> FEGEKVFRVNVEDENDISELHELASTRQIDFWKPDSVTQIKPHSTVDFRVKAEDILAVEDFLEQNELQYEVLINNLRSVLE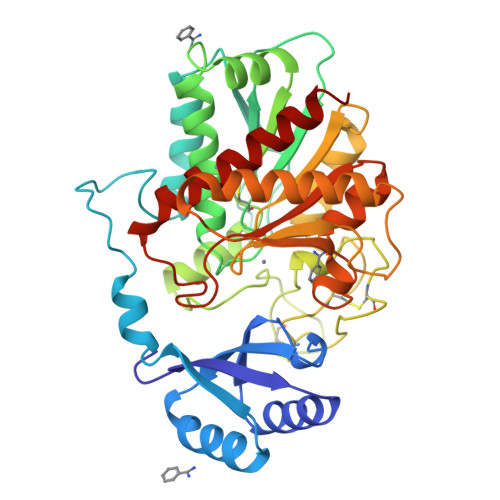AQFDSVSRTTGHSYEKYNNWETIEAWTEQVTSKNPDLISRSAIGTTFDGDNIYLLKVGKPGSNKPAIFMDCGFHAREWISQAFCQWFVRDAVRTYGYEAHMTEFLDNLDFYVLPVLNIDGYIYTWTKNRMWRKTRSTNAGSSCTGTDPNRNFNAGWCTVGASVNPCNETYCGSAAESEKETKALADFIRNNLSSIKAYLTIHSYSQMILYPYSYDYKLPENDAELNSLAKGAVKELASLYGTSYSYGPGSTTIYPAAGGSDDWAYNQGIKYSFTFELRDKGRFGFVLPESQIQATCQETMLAVKYVTNYTLEHL> CGGRARVREYSRAELVIGTLCRVRVYSKRPAAEVHAALEEVFTLLQQQEMVLSAYRDDSALAALNAQAGSAPVVVDRSLYALLERALFFAEKSGGAFNPALGAVVKLWNIGFDRAAVPDPDALKEALTRCDFRQVHLRAGVSVGAPHTVQLAQAGMQLDLGAIAKGFLADKIVQLLTAHALDSALVDLGGNIFALGLKYGDVRSAAAQRLEWNVGIRDPHGTGQKPALVVSVRDCSVVTSGAYERFFERDGVRYHHIIDPVTGFPAHTDVDSVSIFAPRSTDADALATACFVLGYEKSCALLREFPGVDALFIFPDKRVRASAGIVDRVRVLD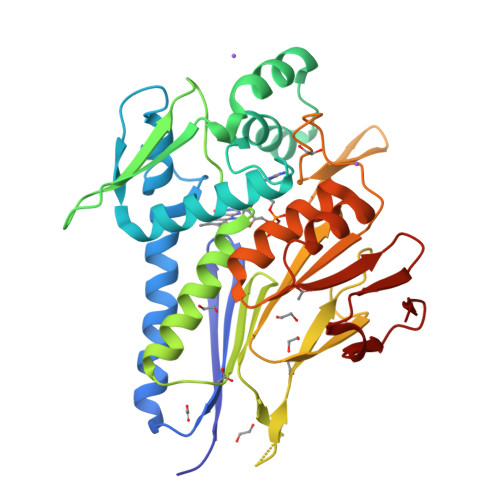ARFVLER> AILGRSETQECLFFNANWERDRTNQTGVEPCYGDKDKRRHCFATWKNISGSIEIVKQGCWLDDINCYDRTDCIEKKDSPEVYFCCCEGNMCN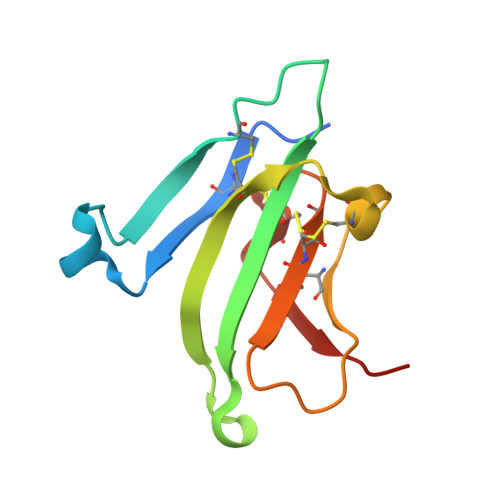EKFSYFPEME>DEEQVFHFYWLDAYEDQYNQPGVVFLFGKVWIESAETHVSCCVMVKNIERTLYFLPREMKIDLNTGKETGTPISMKDVYEEFDEKIATKYKIMKFKSKPVEKNYAFEIPDVPEKSEYLEVKYSAEMPQLPQDLKGETFSHVFGTNTSSLELFLMNRKIKGPCWLEVKSPQLLNQPVSWCKAEAMALKPDLVNVIKDVSPPPLVVMAFSMKTMQNAKN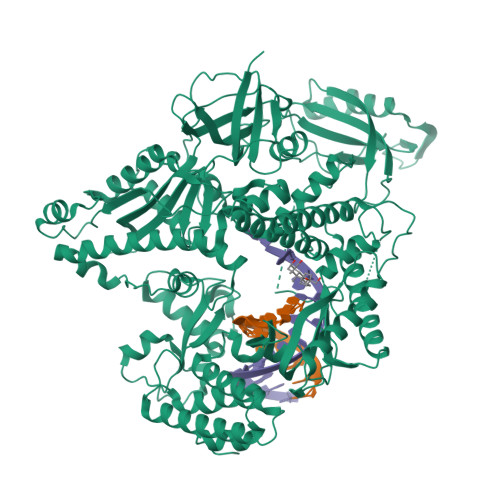HQNEIIAMAALVHHSFALDKAAPKPPFQSHFCVVSKPKDCIFPYAFKEVIEKKNVKVEVAATERTLLGFFLAKVHKIDPDIIVGHNIYGFELEVLLQRINVCKAPHWSKIGRLKRSNMPKLGGRSGFGERNATCGRMICDVEISAKELIRCKSYHLSELVQQILKTERVVIPMENIQNMYSESSQLLYLLEHTWKDAKFILQIMCELNVLPLALQITNIAGNIMSRTLMGGRSERNEFLLLHAFYENNYIVPDKQIFRKPQQKLGDEDEEIDGDTNKYKKGRKKAAYAGGLVLDPKVGFYDKFILLLDFNSLYPSIIQEFNICFTTVQRVASEAQKVTEDGEQEQIPELPDPSLEMGILPREIRKLVERRKQVKQLMKQQDLNPDLILQYDIRQKALKLTANSMYGCLGFSYSRFYAKPLAALVTYKGREILMHTKEMVQKMNLEVIYGDTDSIMINTNSTNLEEVFKLGNKVKSEVNKLYKLLEIDIDGVFKSLLLLKKKKYAALVVEPTSDGNYVTKQELKGLDIVRRDWCDLAKDTGNFVIGQILSDQSRDTIVENIQKRLIEIGENVLNGSVPVSQFEINKALTKDPQDYPDKKSLPHVHVALWINSQGGRKVKAGDTVSYVICQDGSNLTASQRAYAPEQLQKQDNLTIDTQYYLAQQIHPVVARICEPIDGIDAVLIATWLGLDPTQFRVHHYHKDEEN[2x]> MFAIDPLKHSKLYEEYGLYLRPHQINQEIKPTTIKKKELAPTIRSIKYASLIHSMLAKHAARHNGTLINPRMYADMITLGNTKVTVTKGTPKAQIDTLKMNGLTVVSKSRRNNKKKPVSDTTATIDENTDDIVTYKALTEMSTLIESFRLPSGLALIIFDD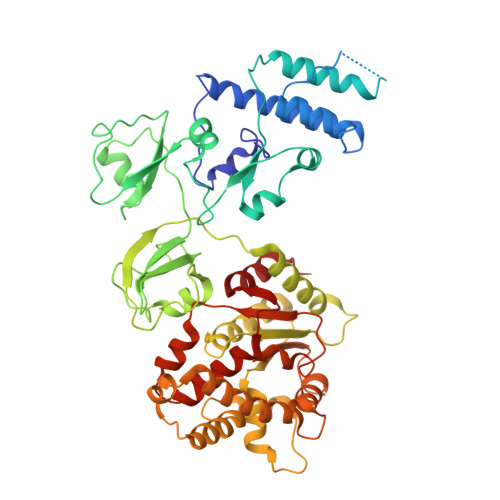EKYQSLIPNYINQLIAYTQPHIIPTWQGIADFSDTYLRSYFKRPFELTASNLAAPQKYNLSPMTRSIFNNTGREDAVIRKLYGYGEYVFIRYEGCLITWTGIYGEVTMMVNLSKRDLGLDVGDDYLKEYKKLLFYGVITDAIPSGISARSTIMKISPHKMMNPSGGALAVLSKFLEAVVSTNVINATLVVYAEKGAGKTSFLSTYAEQLSLASGQVVGHLSSDAYGRWLAKNKDVEEPSFAYDYVLSLDTDDNESYYEQKASELLISHGISEVAQYELLSVRKKIKMMDEMNEVLIAQLENADTHSERNFYYMVSTGKTTPRTLIVEGHFNAQDATIARTDTTVLLRTINDTTQAMRDRQRGGVVQLFLRDTYYRLLPALHTTVYPFEMLESIRRWKWVH> MLRIKEVKKYNNRLGFPAGKEVRIRPLLEAGGFARGPIYVKYGRELSKHDPSSRSMAWNATVFDTALNHPTRPWTVTVVGGKKMVLGVRKEGLGFSEDDPPRSLNVKGGDDMADENYGGGNSTIVLVKSGGKDFAIGLDDLKELNSFGIGAGNGKLSLALGNPVNVLTGVVLPVEQRDGSVAYVAVNSDTKSVIYKVDAKGLQKNQKIDVNVRASAEKILLTKNNELLHISPQGLNVYSVQGSASTFKYFCPYFSSFGGWSRRFVDTVTLMDEGGNQEALIGTGPKGIEYMPVDEKCKNYVVEGVQDAKHAVVAPGATKEGNDIKVLGVYNGELCLLTLEVVDAVEPKLDQGSPAKPSAERVKATKSSKVTVRSGALSKPVSWLRDSLDEASFKNIVDKLSGKIRFSFPLVDLQGRMGLPIKLVVYYDESDGEDMSVLGRHWTLGRDCIVLDHGNTVFEDKQDYYLVKDQMKIRLERDWTKPSANGKVLFNMVGNKDATFEYTAREEKWEVSDGKIRYVYGMNNQGVVSVPGWADWYGPSANYDSKKIHSVQWNLVEISSVAHRDVKLKYTYTPLDPSTHTMHLLSITDDSNKTTIKFSYKTIEGLGKQVSSGLVKEHKFINNKLLEKVEIDSPSTAQVLKLTSTKIDSLYYLESIKQDDDPDPVLGFEYNKDDKLKPRVQQIRLPSKSVVDFKYTKQAIATQQFEQEIAKMADLYTGNEYSLEIEKTVGETDLYVRLKDSAGKNDFIKNQSIRIESYRGFKIKSYSPFMMHSYIAILVRYAEEKEKLHNKIYILNKGEDDSWKLDTTNNNSRVSEDKKFKYDFQEDSFVYYHSKKVHFEYKKSGTKVWSYTSKDIGDVDAFTLMNRGAVYCKNDLVLIRWDALGKLQQETLSDAKSKPSISDVDTFFEYIDVQGTFPEDEAEAKKEVDDYKRDLKESLSDYGLILYNNVVALRTIKLSFTGRITVKVLLYLLKHDYTVSSRSSIELQGGDLAKFNLTLDVFDEHKTKNTNDLDKYRFEFKKQGSKFKLTYIEATDKDNKPTKPSSQNEKLIGQYERRMKIPLDFEKYMMQVNQEGIIVNDHQIIHDNGNFIAKQLDRDTLKLTKFKIPLGAFSNFKKDSDGDEIKLCTKTEQERTESCVSLQTNSARNVSIKYPYYLVTQKKNDIKVLPLKINSRGWEDSVDYRGEILHGSSSHAAMVTTRMSDQKTIVRPLKALNKINKIYAQVISEEKLTTPYDSYVIKYEYEDPVVSMNQVAFKTTIVVPGGGKSATGYYRETNDLQDNQQIVQVMTADNQVFDPEYVKRMNEMQQEEDKQRDGAQLDAEQTITDKSGYHPILKTTPYSANQELVQFLGFEDYEDMTGWTVNKRPIQESNIRRNEFSATGRNFLLLKKGEELIAEFPNTAYYDNFIASTWIRTAQEATVGSTTDMLLLYVDNKPMKGTIKQSIDEWIYVEADSREIVVSESTTVKRVLFKIIVKSTGADDVHVDHVRLSPVNFNFEGSVYDARIGQRTATIQTNGFVSRRLYDAYNRRIAEVDETGNIKYLASYSKRVGNTKDEKKREGGYSSRIQMRAKHSWVESFSPYTMEKRWQIGGTATVEPNQAILQGQIISKEKFSSESICIRLVYSMSGSSQLSLTIGKTTVVVKPNAVQYKGHTATTPSNAELVIFATPKLTSIWVDGHLRIEAPETHAKFNNEAVSLQTSGPVGIKDVIVMEDAEIQVSYLNRDSKPLQEILLLDSSNVLIRQMMYDVIGRRVAETVWVQKS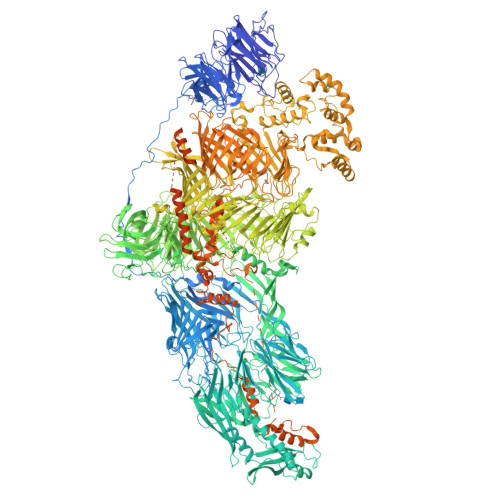LIDGRSTAFKAFQYHDDFVSNDNPTDRNYFLNTGPMQGYVATATNTIYEGYPYSQTVYYNNPLEIRHKVGHPGVKNSIKGAFVHQYAIASDLAFIQRNYPKNEGYRQEEEKSPNGKKHVVVYNRRNKKVAEYTQVKDYNNILTTYIYDQHGNQIQMLPPSYYHEKSRSGDYQPEKQVVASPWAVTSKYDSTGEFITSKETPDGGRVEFIYNEYNQLRYQIHYKEDKQADKIVYFLYNIFGRMCEAGQVPANPTTLQQVRETTKSHQAIPNRDQAVYFDYGETESEPSLRGRIQRTVKKNKEVLFSEVMFFDEESNIIRKSYISPTTNETLSLVYLQENDKVSGIQYPFGVDGKQLILKYKHNLRGEIVEVARVEQKTSGQTEFIPIAGIDHDAEGKVTKISHNYGDSKFDQTYKYVAPGYLVEIANNFLTEKLYYTEKGYGCEPTGDGSILRTEFKASWHDKCDQNLIPLTARAFVSGGIDFTTAETCFDALLNLGYIDTTGRPVKTFYPDLETGLPMKCATPSNWRYISEKMLEQGYPEHYGHAYDYGSHGELIAAKSFVGKEKDSLTAPLSKASFANAGMKSHELDRFWDSLSRSINKVEGTKAIFEGTQQLTTGLVGSVIHKPKLESLLEGKGGDSSICTPWSSGDRTEEAKCKREYQQAFDKLKLKQVIQSLQEPVRKNVLRILKNTLASMLGNSPGDVESFSIDPNGNHGVFYTGFKRFELKYKHQKNQIATIKEGTKQQEKMIVHDDEGNVIKALHKKIDKIEYDPLTQRVSRIEMSDRSRTLEFGYDFRGERTFKRVRNKDNDIISVNYYVRDNKGNVLVEYKQEYPNPKDTNKPINTVTAYIHGPLGLLGFFRNNKYYNVLLDHEGSTRLVIHQGKVVAAYDYLPYGQMIRKYGSNPEAHIAFRYTGQEFDEETGLYNYHARLYDPDIGRFFQMDPMEQYASPYKYAGNSPVSQIDPDGQIAVTLVLMIIGAIVGAYLGAASANNSWNPAKWAWGDKKTWIGLFAGAIMGAFAVYGGAATFSYFTAMFGGSMIAGALATGVISVAGAFLGAAAASNQWNPAKWDWTSPAVWNGLLSGASIAVSFPSGFVGITRSFMSISSNLVKMIYASLMVGGFLLFVYLGGGMANNFNFQISQWDWKSPRTWFGMIEGASTIFMGTAGTAKHGAAKVYNVVKPNGLKMIWHKVNIPSKAFTMRRVKDTIILTWYKNGQSISKQILKTTVKADLAKIPKDFIMIHRGFFMPYQRIGYAAIAMPSMAGLMFKKNQYFFTNHPNGTLTKHVRKKRSAPMSSSAASPSVSNFLNDFFENMSELFDSFFSQTEHSHQDSQSSLSIGASYGRPSNESYHKSFQKLCYSPDSDGNQIICPQRESTVNIFSKGETFAPEAFGQDLFSRCLPLTWHDRPSIACDGEQTTFIYTPNQNIRVFDMVDGWLMLARIAPAALRNLKAGFSFLRDVVFSDEREQTVQVNDLSRCKQDLEVELLDLKRVMLKKQPNEVKWAQPILNDLEDDIGEFLSERKPSEKEFELLQERLSALREEIMENSSVATELNLSTLIGDMLKKMDGVNVGLNGDVRDMISTLSGMVPFSSSNLLA>[2x]MGPDDYVPSQIAVNTSTLPGVVIGPADAHTYPRVIGELAGTSNQYVFNGGAIALMRGKFTPALPKIGSITYTFHQGNSRDSSD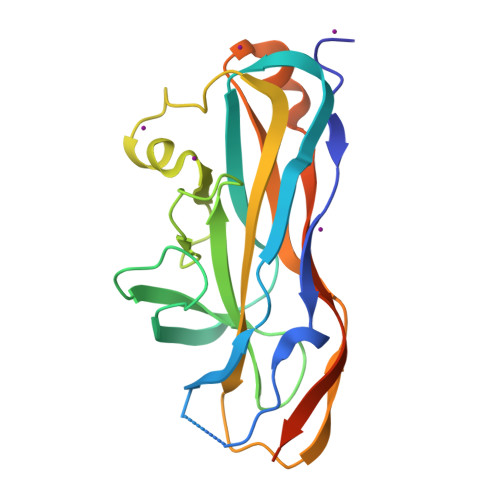FDIYDIGVSGLGIIIGMAGYWPATPLVPINSSGIYIDPVGANTNPNTYNGATASFGARLFVAFVATGRLPNGYITIPTRQLGTILLEAKRTSLNNKGLTAPVMLNGGRIQVQSQTCTMGLEHHHHHH> GSGSGKPAPDAIGDLLASVDSEEVRQYC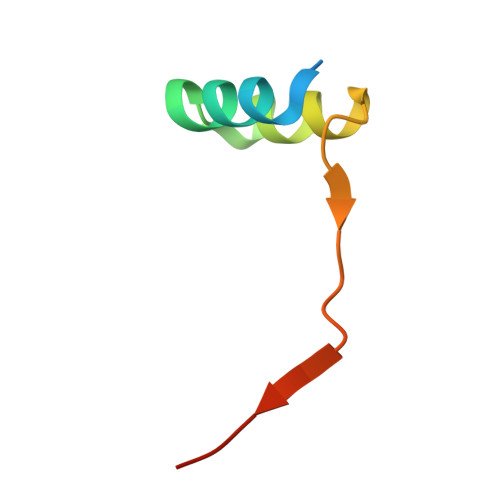REQGWIIPETPTNVERHLNR> SRKIIHVDMDCFAAAVEMRDNPALRDIPIAIGGSRERRGVISCANYPARKFGVRSAMPTGMALKLCPHLTLLPGRFDAYKEASNHIREIFSRYTSRIEPLSLDEAYLDVTDSVHCHGSATLIAQEIRQTIFNEL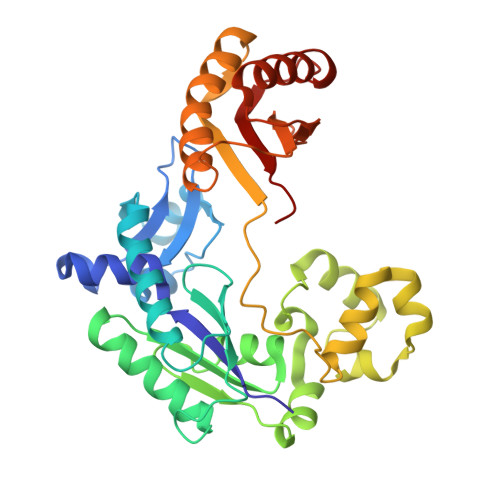QLTASAGVAPVKFLAKIASDMNKPNGQFVITPAEVPAFLQTLPLAKIPGVGKVSAAKLEAMGLRTCGDVQKCDLVMLLKRFGKFGRILWERSQGIDERDVNSERLRKSVGVERTMAEDIHHWSECEAIIERLYPELERRLAKVKPDLLIARQGVKLKFDDFQQTTQEHVWPRLNKADLIATARKTWDERRGGRGVRLVGLHVTLLDP> SNAMENEKILNPIIIQRADPMIYKHNDGYYYFTASVPEYDRIEVRKAKTIEGLRNAEPVDVWRRHESGEMSNLIWAPEIHFINGAWYIYFAAAPDKNIEDDTFNHRMFVIQNENENPFTGNWVEKGRIKTAWESFSLDATIFEHNEKLYYVWAQQDINIKGHSNIYIAEMENPWTLKTKPVMLTKPELEWEIKGFWVNEGPAVLKKNGKIFITYSA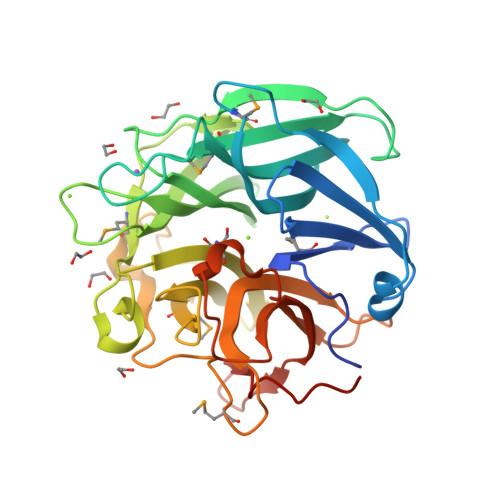SATDVNYCIGMLTAEENSNLLDKNSWTKSQTPVFKTSMENHQYGPGHNSFTVSEDGKHDVIVYHARNYTEIKGDPLYDPNRHTRAQIINWREDGTPDFGVPEVDSLEIETPVKA> GSGAPPTDLQKMVMGNTKPVELILDGKTVAICCATGVFGTAYLVPRHLFAEKYDKIMLDGRAMTDSDYRVFEFEIKVKGQDMLSD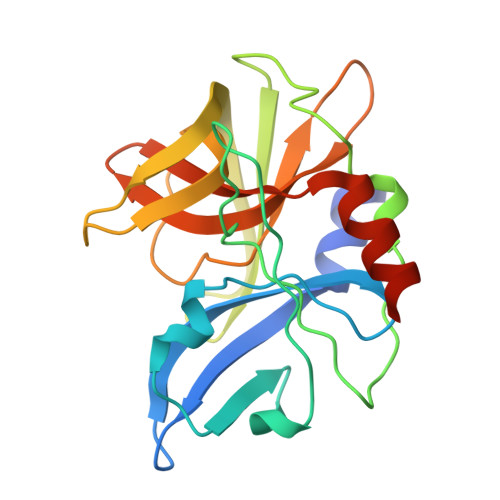AALMVLHRGNKVRDITKHFRDTARMKKGTPVVGVVNNADVGRLIFSGEALTYKDIVVLMDGDTMPGLFAYKAATRAGYAGGAVLAKDGADTFIVGTHSAGGNGVGYCSCVSRSMLQKMKAHVDPEPHHE> MMFNKQIFTILILSLSLALAGSGCISEGAEDNVAQEITVDEFSNIRENPVTPWNPEPSAPVIDPTAYIDPQASVIGEVTIGANVMVSPMASIRSDEGMPIFVGDRSNVQDGVVLHALETINEEGEPIE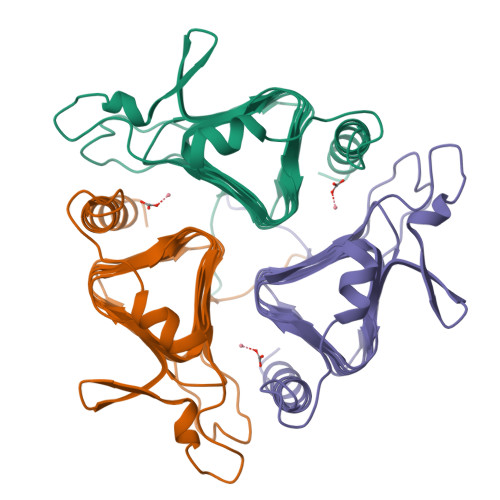DNIVEVDGKEYAVYIGNNVSLAHQSQVHGPAAVGDDTFIGMQAFVFKSKVGNNCVLEPRSAAIGVTIPDGRYIPAGMVVTSQAEADKLPEVTDDYAYSHTNEAVVYVNVHLAEGYKETS>MTQAIKRVGVTDVVLRDAHQSLFATRLRIDDMLPIAQQLDQIGYWSLECWGGATFDSCIRFLGEDPWQRLRLLKQAMPNTPLQMLLRGQNLLGYRHYADDVVDTFVERAVKNGMDVFRVFDAMNDVRNMQQALQAVKKMGAHAQGTLCYTTSPVHNLQTWVDVAQQLAELGVDSIALKDMAGILTPYAAEELVSTLKKQVDVELHLHCHSTAGLADMTLLKAIEAGVDRVDTAISSMSGTYGHPATESLVATLQGTGYDTGLDIAKLEQIAAYFRDVRKKYHAFEGMMKGSDARILVAQVPGGMLTNMESQLKQQNALDKLDLVLEEIPRVREELGFLPLVTPTSQIVGTQAVINVVLGERYKTITKETSGVLKGEYGKTPAPVNTELQARVLAGAEAITCRPADLIAAEMPTLQDRVLQQAKEQHI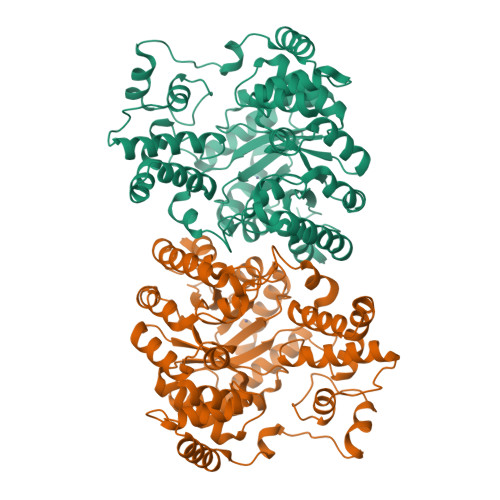TLAENAIDDVLTIALFDQVGWKFLANRHNLEHHHHHH[2x]> MKKISRKEYVSMYGPTTGDKVRLGDTDLIAEVEHDYTIYGEELKFGGGKTLREGMSQSNNPSKEELDLIITNALIVDYTGIYKADIGIKDGKIAGIGKGGNKDMQDGVKNNLSVGPATEALAGEGLIVTAGGIDTHIHFISPQQIPTAFASGVTTMIGGGTGPADGTNATTITPGRRNLKWMLRAAEEYSMNLGFLAKGNTSNDASLADQIEAGAIGFKIHEDWGTTPSAINHALDVADKYDVQVAIHTDTLNEAGCVEDTMAAIAGRTMHTFHTEGAGGGHAPDIIKVAGEHNILPASTNPTIPFTVNTEAEHMDMLMVCHHLDKSIKEDVQFADSRIRPQTIAAEDTLHDMGIFSITSSDSQAMGRVGEVITRTWQTADKNKKEFGRLKEEKGDND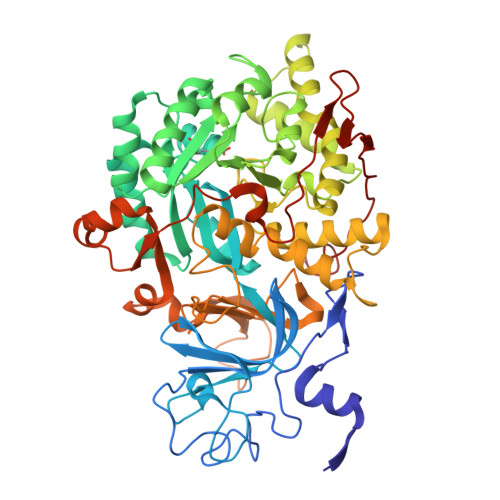NFRIKRYLSKYTINPAIAHGISEYVGSVEVGKVADLVLWSPAFFGVKPNMIIKGGFIALSQMGDANASIPTPQPVYYREMFAHHGKAKYDANITFVSQAAYDKGIKEELGLERQVLPVKNCRNITKKDMQFNDTTAHIEVNPETYHVFVDGKEVTSKPANKVSLAQLFSIF>MLVSVYLALLVACVGQAHSQANLMRLKSDLFNRSPMYPGPTKDDPLTVTLGFTLQDIVKVDSSTNEVDLVYYEQQRWKLNSLMWDPNEYGNITDFRTSAADIWTPDITAYSSTRPVQVLSPQIAVVTHDGSVMFIPAQRLSFMCDPTGVDSE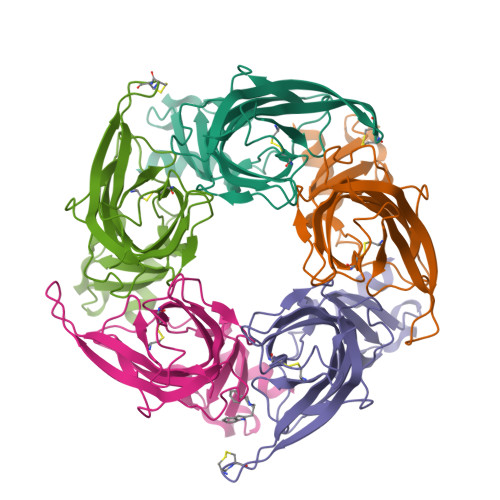EGVTCAVKFGSWVYSGFEIDLKTDTDQVDLSSYYASSKYEILSATQTRQVQHYSCCPEPYIDVNLVVKFRERRAGNGFFRNLFD[5x]> MEVHEEQVSAPVTGDATAKYLLQYILSARGICHENALILALMRLETDASTLNTEWSIQQWVDK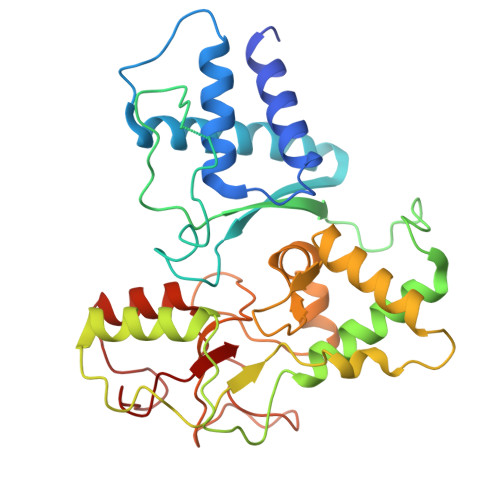LNDYINAINVKLNLLGYKIIRINHGIGRNAVTLKAKQNFESFEDNTAIRAHNNDYAVLQSIVLPESNRFFVYVNLASTEETKLATRFNQNEIEFMKWAIEQFMISGETIVEGPALETSIIVKEVNRILVAATGDSNLAKWRKFSTFTVGSTNLFQFQELTATDIEDLLLRLCELKWFYRTQEGKFGIDLRCIAELEEYLTSMYNLNTCQNCHKLAIQGVRCGNESCREENEETGENSLSQIWHVDCFKHYITHVSKNCDRCGSSLITEGVYVI>MFTGLVETTGKILEIQETNEGRGFLVET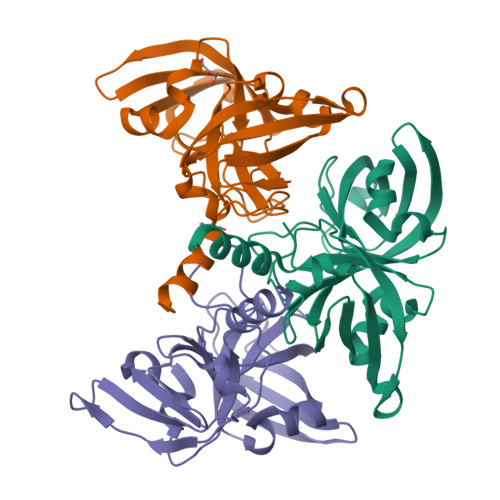KWVQPDLKLGDSISVNGCCQTVTEFTNEGSRFRFYASFKTLELTNFKFLKVGEEVNLERSALPTTRLGGHLVSGHVDGTGKILSKEEREGGAVICYTVQNDPSLSRYIAPRGSITVDGISLTVVDSRPKEFDLVLIPETLKKTNAKSWNSDTILNLEIDLVARYLEQLLKSKELVPRGSLE[3x]> MRAVNWNKKEDDFSLMFWKQNIAQFWTEEEIAVSSDKNTWVQLSKEEQIAYK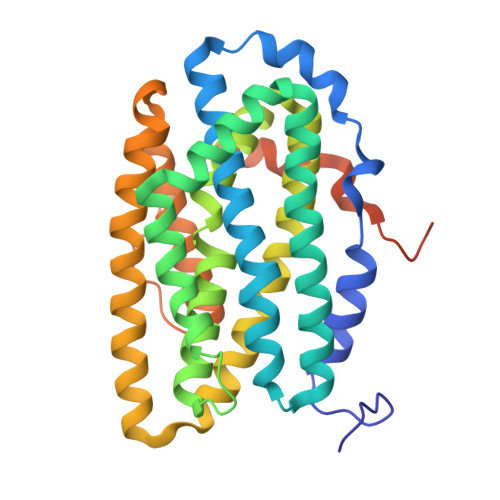RVLGGLTLLDTKQGGEGMPLVLVHLENLQAKSVLAFMGAMEEVHAKSYSHIFTTLATEEEIDDIFDWVDNHPLLEKKAGIITSYYRRLLKPEVTKKELYMAMVASVFLESYLFYSGFFYPLYLAGQGKLTASGEIINLIIRDESIHGVFVGILAQQIFAELSAEEQQEVQKETQELLMELYEIEMAYTEEIYTSIGLVEDVNRFVRYNANKGLMNLGLEPKFEEEEINPIVLNGLRTDTKNHDFFSVKGNGYVKATNVEKLADDDFVFNF>MKVVYDDVRVLKDIIQALARLVDEAVLKFKQDSVELVALDRAHISLISVNLPREMFKEYDVNDEFKFGFNTQYLMKILKVAKRKEAIEIASESPDSVIINIIGSTNREFNVRNLEVSEQEIPEINLQFDISATISSDGFKSAISEVSTVTDNVVVEGHEDRILIKAEGESEVEVEFSKDTGGLQDLEFSKESKNSYSAEYLDDVLSLT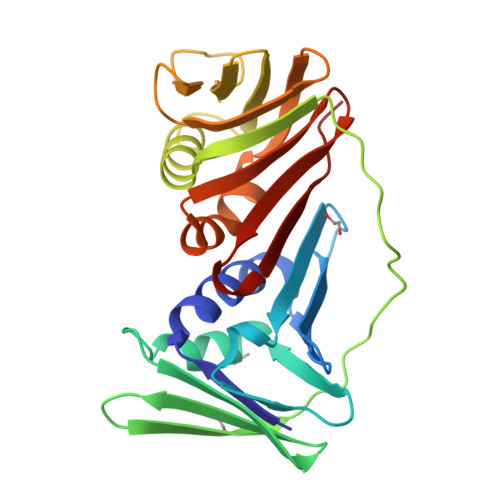KLSDYVKISFGNQKPLQLFFNMEGGGKVTYLLAPKV[4x]> MISLVFVLLIGAAFATEDDKIVGGYECKPYSQPHQVSLNSGYHFCGGSLVNENWVVSAAHCYKSRVEVRLGEHNIKVTEGSEQFISSSRVIRHPNYSSYNIDNDIMLIKLSKPATLNTYVQPVALPTSCAPAGTMCTVSGWGNTMSSTADSNKLQCLNIPILSYSDCNNSYPGMITNAMFCAGYLEGGK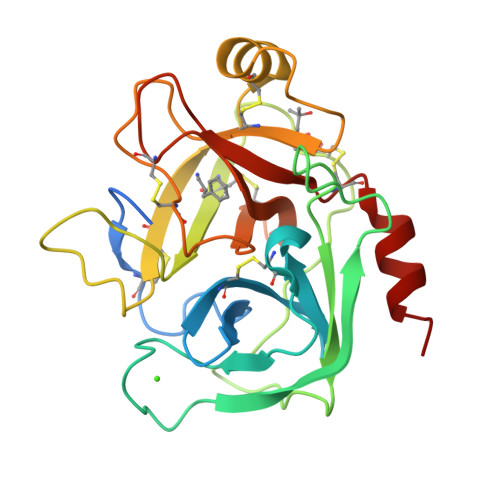DSCQGDSGGPVVCNGELQGVVSWGYGCAEPGNPGVYAKVCIFNDWLTSTMASY> LPTPVGMEIMPPQPPLPPDSSSQDCDPTASLRPFATKAEADAAVADIRARGRLIVGLDIGSNLFSFRDPITGEITGFDVDIAGEVARDIF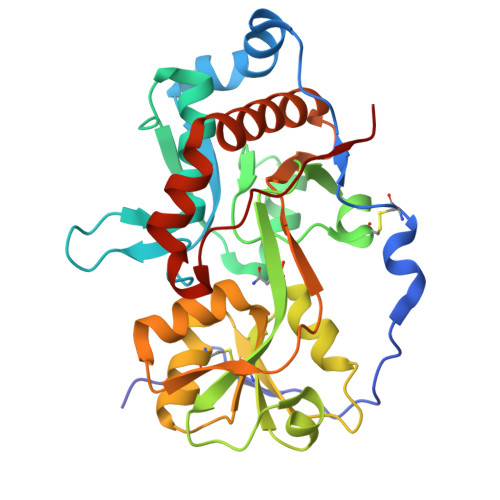GVPSHVEYRILSAAERVTALQKSQVDIVVKTMSITCERRKLVNFSTVYLDANQRILAPRDSPITKVSDLSGKRVCVARGTTSLRRIREIAPPPVIVSVVNWADCLVALQQREIDAVSTDDTILAGLVEEDPYLHIVGPDMADQPYGVGINLDNTGLVRFVNGTLERIRNDGTWNTLYRKWLTVLGPAPAPPTPRYVD> GSSIKQRTLKNIIRATGVGLHSGEKVYLTLKPAPVDTGIVFCRTDLDPVVEIPARAENVGETTMSTTLVKGDVKVDTVEHLLSAMAGLGIDNAYVELSASEVPIMDGSAGPFVFLIQSAGLQEQEAAKKFIRIKREVSVEEGDKRAVFVPFDGFKVSFEIDFDHPVFRGRTQQASVDFSSTSFVKEVSRARTFGFMRDIEYLRSQNLALGGSVENAIVVDENRVLNEDGLRYEDEFVKHKILDAIGDLYLLGNSLIGEFRGFKSGHALNNQLLRTLIADKDAWEVVT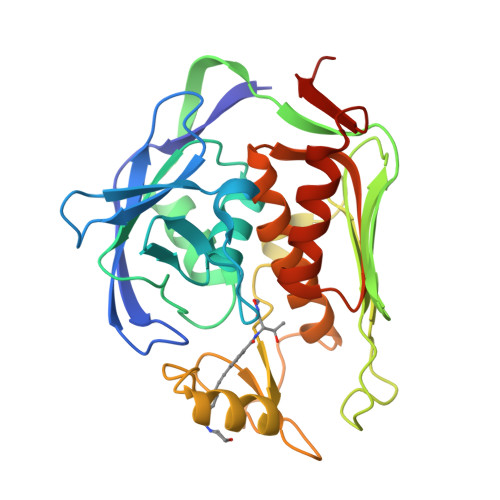FEDARTAP>MEGRLLLLETPGNTRMSLAYDEAIYRSFQYGDKPILRFYRHDRSVIIGYFQVAEEEVDLDYMKKNGIMLARRYTGGGAVYHDLGDLNFSVVRSSDDMDITSMFRTMNEAVVNSLRILGLDARPGELNDVSIPVNKKTDIMAGEKKIMGAAGAMRKGAKLWHAAMLVHTDLDMLSAVLKVPDEKFRDKIAKSTRERVANVTDFVDVSIDEVRNALIRGFSETL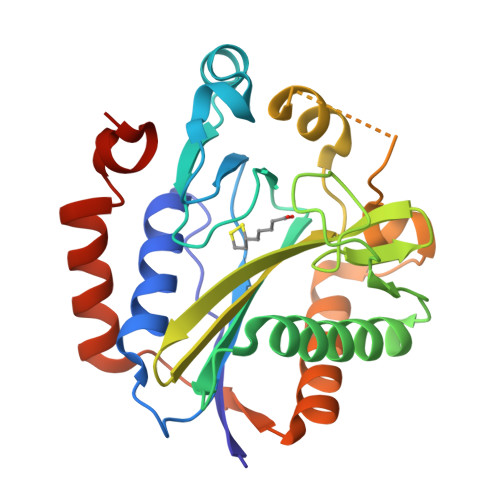HIDFREDTITEKEESLARELFDKKYSTEEWNMGLLRKEVV[4x]The xylan-specific α-glucuronidases from glycoside hydrolase family 115 (GH115) specifically catalyse the removal of α-d-glucuronic acid (GlcA) or methylated GlcA (MeGlcA). In this study, we report crystal structures of a bacterial GH115 ortholog (wtsAgu115A) identified in a metagenome from an anaerobic digester fed with wastewater treatment sludge. Furthermore, wtsAgu115A eluted from a gel-filtration column at a volume consistent with a dimer in solution, which suggests that wtsAgu115A is a dimer in its active form similar to other GH115 xylan-specific α-glucuronidases.

A crystal structure at 2.65 Å resolution of wtsAgu115A originating from a metagenome from an anaerobic digester fed with wastewater treatment sludge was determined in complex with xylohexaose, and Asp303 was identified as the likely general acid. The sum of φ and ψ for the glycosidic linkages between the xylose moiety pairs at +2NR and +1NR, at +1NR and +1, at +1 and +1R and at +1R and +2R are 47°, 27°, 57° and 13°, respectively, which indicates that the xylan backbone is forced out of conformation upon forming the Michaelis–Menten complex. The xylohexaose-bound crystal structure forms a Michaelis–Menten-like complex, which reveals how the dimer interface of the enzyme orients xylan in the active site guided by residues from each protomer of the homodimer. If this were the case, a distant residue could activate the active-site water nucleophile, which was also suggested to be the case for cellulases in glycoside hydrolase family 6. The wtsAgu115A–xylohexaose structure revealed a proton wire leading from Ca2+ site 1 to Tyr403 through the active-site cavity via water molecules w427, w446 and w484 (see Supplementary Fig. S6 for an omit map) and likely beyond Ca2+ site 1. Thus, the proton required for catalysis could be delivered through this proton wire. Interestingly, upon formation of the Michaelis–Menten-like complex, Tyr403 moved nearly 170° and the nearby histidine residues His246 and His247 also underwent conformational changes, indicating the importance of Tyr403 in particular in catalysis.

> AGDNKGITYEELNPERFTLLEKGTPTNILIDENEDQGVMIAATNLSEDFGRVSGTNAPLIFLPDNERLIIVGTLESRYIKELTENRKIKGDELKGKNEKYLMTVVDNPLPGVKEALIIAGSDKRGAIYGIYELSEQIGVSPWYDWADVPVKPQQNLSIERGSYTADEPAVTYRGIFLNDEAPALTSWVENTYGTKYGDHRFYSRVFELILRLRGNFLWPAMWDWSFYGDDPLNSKTADTMGIIMGTSHHEPMARNHQEWARNRDKYGVWDYTSNQEVIDQFFREGIERVKDTDDLITIGMRGDGDTPMPMGVKEGEDHLPSDEDNMRLLERIIKNQREIIGDVTGESPEKTPQVWAIYKEVQRYFDLGLRPPEDVIILLSDDNWGNVRRLPTEEERDHPGGWGMYYHFDYVGAPRSSKWLNISPIQNIWEQMQLTYDYGVDELWVANVGDLKPMEYPITLFLDMAWDPTRFNAENLLDHTRSFAAQQFGEDQADEAARIINLYSKYNGRVTPEMLDRNTYNLESGEWKKVSDEYIKLEAEALRQYLTLEPEQRDAYKQLILYPVQAMANLYEMYYSQAMNHKLYRENNPMANYWADRVEETFNRDAELSHDYNKVMANGKWDGMMTQKKIGYRSWNDNFPADTLPQIFRIENPEEATGGYVFTARDGVVVIEAEHYFEAKDAEEAKWTVIPYMGRTLSSIALMPYTKEVEGASLSYRMQIPDEVSEVKVHVVVKSTLPFHDPKGHEYRVGFEGGSKEIVNFNWNLNEEPENIYSVFYPTVASRVVKKDVTLDLHDTDDGFYTLTLEPLDPGIVFQKIVVDFGGYEESRLFMEESPNKRIEIE> MERYENLFAQLNDRREGAFVPFVTLGDPGIEQSLKIIDTLIDAGADALELGVPFSDPLADGPTIQNANLRAFAAGVTPAQCFEMLALIREKHPTIPIGLLMYANLVFNNGIDAFYARCEQVGVDSVLVADVPVEESAPFRQAALRHNIAPIFICPPNADDDLLRQVASYGRGYTYLLSRSGVTGAENRGALPLHHLIEKLKEYHAAPALQGFGISSPEQVSAAVRAGAAGAISGSAIVKIIEKNLASPKQMLAELRSFVSAMKAASRA;> TTLLNPYFGEFGGMYVPQILMPALNQLEEAFVRAQKDPEFQAQFADLLKNYAGRPTALTKCQNITAGTRTTLYLKREDLLHGGAHKTNQVLGQALLAKRMGKSEIIAETGAGQHGVASALASALLGLKCRIYMGAKDVERQSPNVFRMRLMGAEVIPVHSGSATLKDACNEALRDWSGSYETAHYMLGTAAGPHPYPTIVREFQRMIGEETKAQILDKEGRLPDAVIACVGGGSNAIGMFADFINDTSVGLIGVEPGGHGIETGEHGAPLKHGRVGIYFGMKAPMMQTA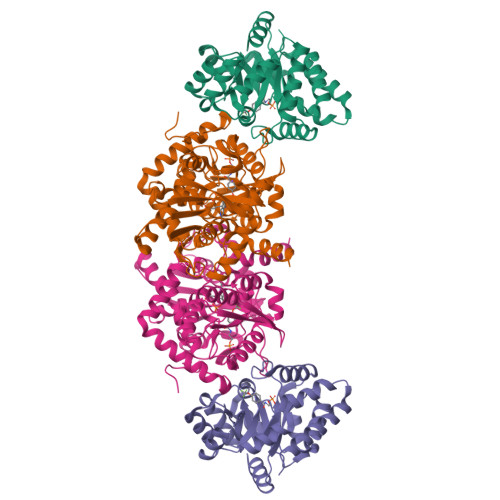DGQIEESYSISAGLDFPSVGPQHAYLNSIGRADYVSITDDEALEAFKTLCRHEGIIPALESSHALAHALKMMREQPEKEQLLVVNLSGRGDKDIFTVHDILKARGEI> SWLLRLFESKLFDISMAISYLYNSKEPGVQAYIGNRLFCFRNEDVDFYLPQLLNMYIHMDEDVGDAIKPYIVHRCRQSINFSLQCALLLGAYSSDMHISTQRHSRGTKLRKLILSDELKPAHRKRELPSLSPAPDTGLSPSKRTHQRSKSDATASISLSSNLKRTASNPKVENEDEELSSSTESIDNSFSSPVRLAPER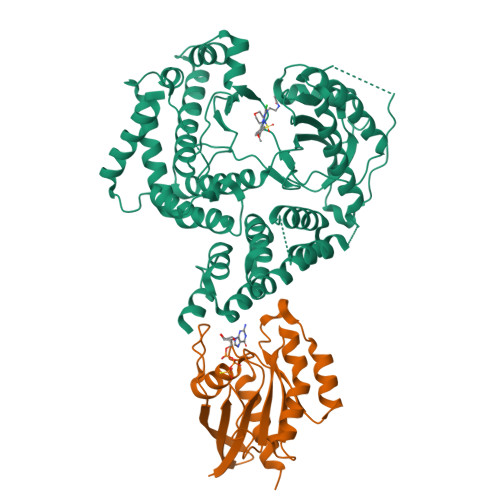EFIKSLMAIGKRLATLPTKEQKTQRLISELSLLNHKLPARVWLPTAGFDHHVVRVPHTQAVVLNSKDKAPYLIYVEVLECENFDTTSVPARIPENRRDPEDPSAVALKEPWQEKVRRIREGSPYGHLPNWRLLSVIVKCGDDLRQELLAFQVLKQLQSIWEQERVPLWIKPYKILVISADSGMIEPVVNAVSIHQVKKQSQLSLLDYFLQEHGSYTTEAFLSAQRNFVQSCAGYCLVCYLLQVKDRHNGNILLDAEGHIIHIDFGFILSSSPRNLGFETSAFKLTTEFVDVMGGLDGDMFNYYKMLMLQGLIAARKHMDKVVQIVEIMQQGSQLPCFHGSSTIRNLKERFHMSMTEEQLQLLVEQMVDGSMRS;> GAMGSMGTRDDEYDYLFKVVLIGDSGVGKSNLLSRFTRNEFNLESKSTIGVEFATRSIQVDGKTIKAQIWDTAGQERYRAITSAYYRGAVGALLVYDIAKHLTYENVERWLKELRDHADSNIVIMLVGNKSDLRHLRAVPTDEARAFAEKNGLSFIETSALDSTNVEAAFQTILTEIYRIVSQKQMSDRRENDMSPSNNVVPIHVPPTTENKPKVQCCQNI>[2x]EREALPPQKIEVLVLLPQDDSYLFSLTRVRPAIEYALRSVEGNGTGRRLLP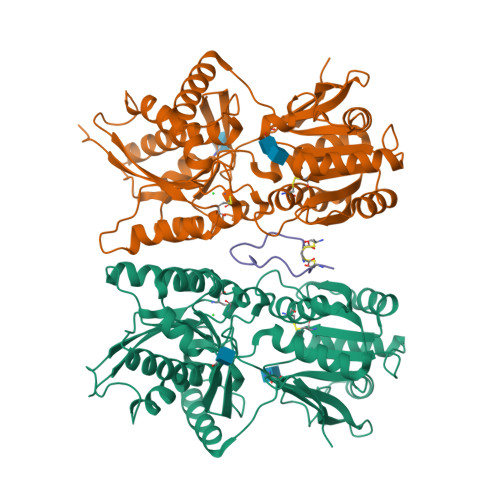PGTRFQVAYEDSDCGNRALFSLVDRVAAARGAKPDLILGPVCEYAAAPVARLASHWDLPMLSAGALAAGFQHKDSEYSHLTRVAPAYAKMGEMMLALFRHHHWSRAALVYSDDKLERNCYFTLEGVHEVFQEEGLHTSIYSFDETKDLDLEDIVRNIQASERVVIMCASSDTIRSIMLVAHRHGMTSGDYAFFNIELFNSSSYGDGSWKRGDKHDFEAKQAYSSLQTVTLLRTVKPEFEKFSMEVKSSVEKQGLNMEDYVNMFVEGFHDAILLYVLALHEVLRAGYSKKDGGKIIQQTWNRTFEGIAGQVSIDANGDRYGDFSVIAMTDVEAGTQEVIGDYFGKEGRFEMRPNVKYPWGPLKLRIDENRIVEHTNSSPCKSCGLEESAVT;> GLSKGCFGLKLDRIGSMSGLGC> GSGGSGKVVKFSYMWTINNFSFCREEMGEVIKSSTFSSGANDKLKWCLRVNPKGLDEESKDYLSLYLLLVSCPKSEVRAKFKFS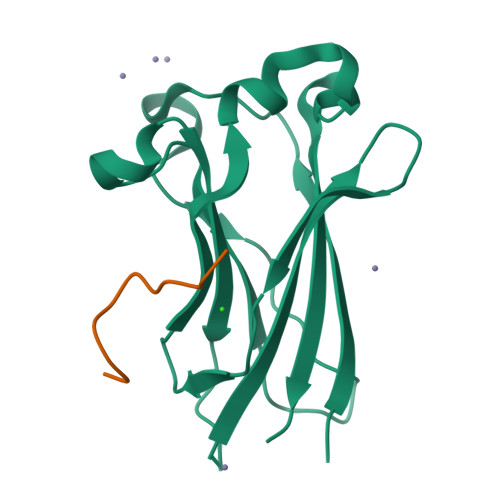ILNAKGEETKAMESQRAYRFVQGKDWGFKKFIRRDFLLDEANGLLPDDKLTLFCEVSVVQD;> KAASADSTTEGTPAD5-azanyl-3,6-dihydro-[1,2,3]triazolo[4,5-d]pyrimidin-7-one | C4 H4 N6 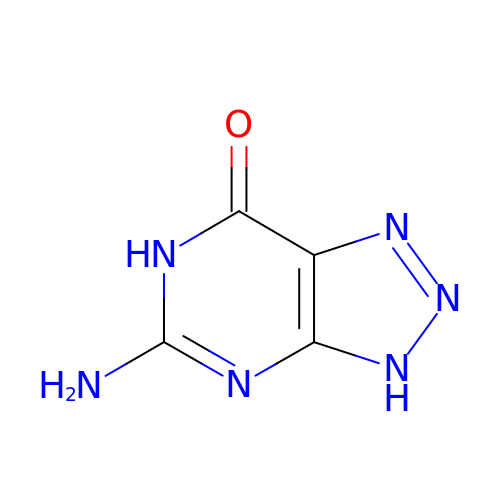O | LPXQRXLUHJKZIE-UHFFFAOYSA-N Di-glutathione-PhenylArsine | C26 H37 As N6 O12 S2 | 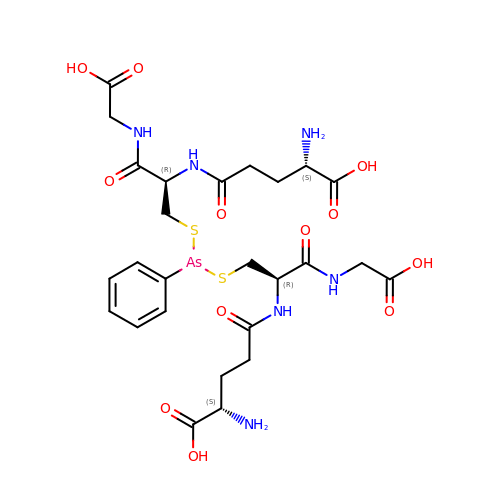PIQQHKNUDQAGPN-XSLAGTTESA-N>SNATGFLVSFMVDARGGSMRG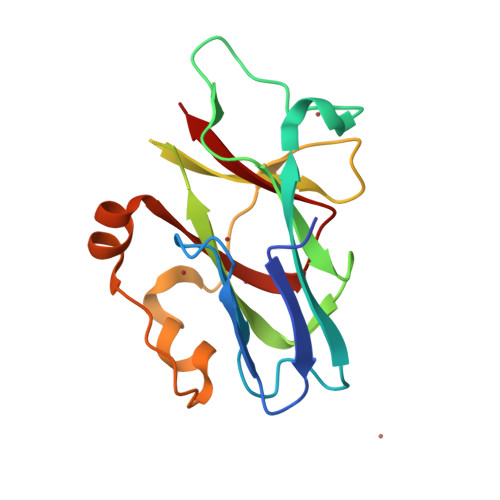SRHNGLRVVIPPRTCAAPTRITCRLVKPQKLSTPPPLAEEEGLASRIIALGPTGAQFLSPVIVEIPHFASHGRGDRELVVLRSENGSVWKEHRSRYGESYLDQILNGMDEELGSLEELEKKRVCRIITTDFPLYFVIMSR[4x]N-decanoyl-L-homoserine | C14 H27 N O4 | 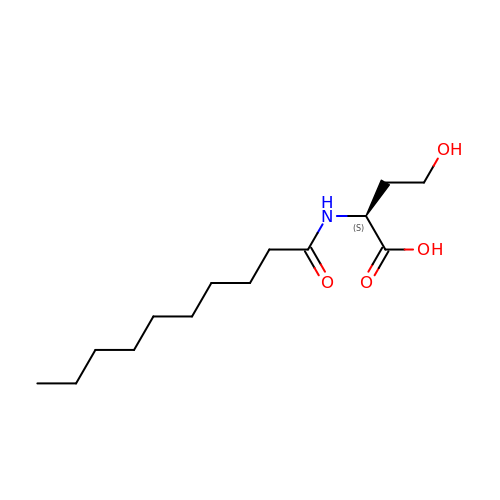SRVJGOTYLHNRPN-LBPRGKRZSA-N>[4x]MDSLDQCIVNACKNSWDKSYLAGTPNKDNCSGFVQSVAAELGVPMPRGNANAMVDGLEQSWTKLASGAEAAQKAAQGFLVIAGLKGRTYGHVAVVISGPLYRQKYPMCWSGSIAGAVGQSQGLKSVGQVWNRTDRDRLNYYVYSLASCSLPRASLEHHHHHH

Members of the bacterial T6SS amidase effector (Tae) superfamily of toxins are delivered between competing bacteria to degrade cell wall peptidoglycan. We focused on Tae1 (previously known as Tse1) from the common soil bacterium Pseudomonas aeruginosa, which is known to interact with a wide range of microbes, including E. coli. The taes encode hydrolase enzymes that induce recipient cell lysis by breaking down the major structural component of bacterial cell envelopes, PG. Furthermore, Tae1 injected into nearby kin cells is deactivated through binding by a cognate immunity protein, T6S amidase immunity protein 1 (Tai1), preventing lysis.

We were particularly struck by one variant, Tae1C110S, which is modified at a partially buried residue sitting directly behind the catalytic Cys30 site. The Cys110Ser substitution was the top-scoring GOF variant in the D-Met screen and ranked 11th amongst GOF variants in the M9 screen. Using the E. coli lysis assay, we first confirmed that Tae1C110S indeed lysed cells at a faster rate than Tae1WT in cells grown in both D-Met and M9 minimal media. We did not observe any major structural rearrangements that would immediately implicate distinct modes of Tai1PA-binding (RMSD = 0.746). However, we did observe some key side chain alterations near the Tae1C110S active site, which is the enzyme region most intimately engaged with Tai1PA upon binding. Most notably, we found that His91 protruded away from the active site of Tae1C110S, which would sterically clash with a loop of Tai1PA that typically inserts into the catalytic cleft. Our structural observations are consistent with the hypothesis that the Cys110 position is important for Tai1 recognition; therefore, serine at this position in P. aeruginosa may be disfavored to preserve immunity to the toxin. We measured Tai1-binding affinity (Kd) for recombinant Tae1WT and Tae1C110S proteins by isothermal titration calorimetry and found that Tae1WT bound Tai1 with ~36-fold greater affinity than Tae1C110S (9.5 nM Kd and 349.6 nM Kd, respectively). Indeed, for PAC110S we observed substantially reduced growth compared to PAWT on solid media but not in liquid media, where T6S is not induced. This phenotype strongly suggests that Tae1C110S lyses kin cells at a faster rate than Tai1 can bind and inhibit killing, leading to a fitness cost for this strain.>SNAEKWTSTAIITQPDVGQIAGYNNAMNVIYGQAAPKVSDLQETLIGRFSSAFSALPETLDNQEEPEKLTIEPSVKNQQLPLTVSYVGQTAEGAQMKLAQYIQQVDDKVNQELEKDLKDNIALGRKNLQDSLRTQEVVAQEQKDLRIRQIQEALQYANQAQVTKPQVQQTEDVTQDTLFLLGSEALESMIKHEATRPLVFSPNYYQTRQNLLDIEKLKFDDLDIHAYRYVMKPTLPIRRDS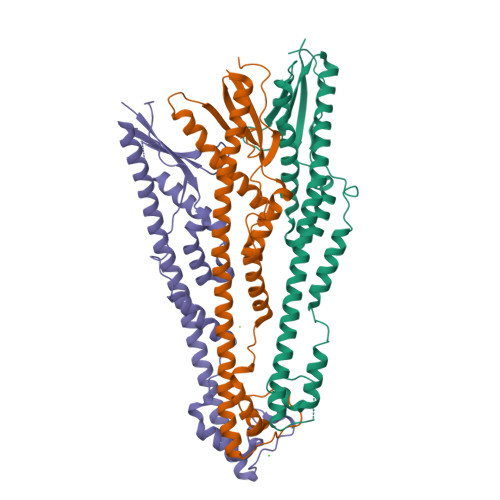PK[3x]>[2x]MHHHHHHMSGGLTPDQAIDAIRGTGGAQPGCRALHAKGTLYRGTFTATRDAVMLSAAPHLDGSTVPALIRFSNGSGNPKQRDGAPGVRGMAVKFTLPDGSTTDVSAQTARLLVSSTPEGFIDLLKAMRPGLTTPLRLATHLLTHPRLLGALPLLREANRIPASYATTEYHGLHAFRWIAADGSARFVRYHLVPTAAEEYLSASDARGKDPDFLTDELAARLQDGPVRFDFRVQ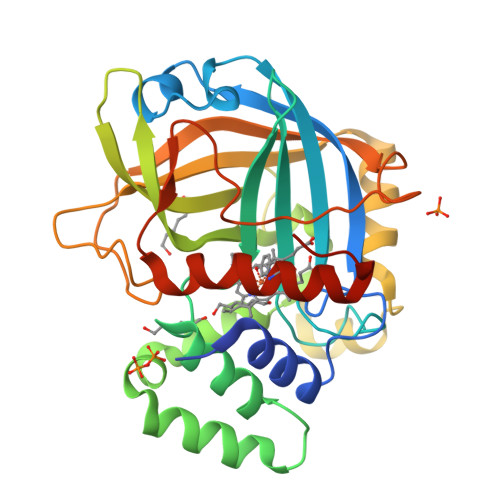IAGPTDSTVDPSSAWQSTQIVTVGTVTITGPDTEREHGGDIVVFDPMRVTDGIEPSDDPVLRFRTLVYSASVKLRTGVDRGAQAPPV> MKQECNVCYFNLPDPE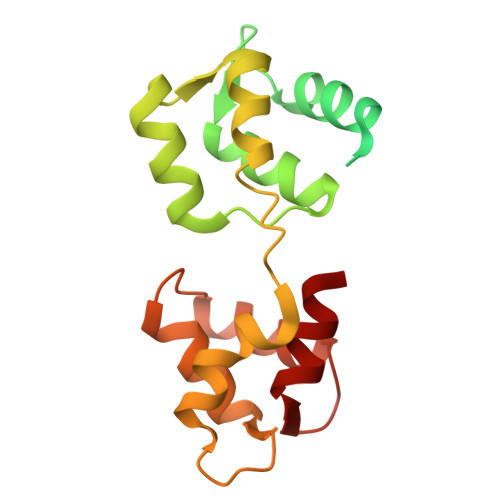STLGPYDNELNYFTWGPGFEYEPEPQRKPLSIEESFENSEESEESVADIQQLEEKVDESDVRIYFNEKSSGGKISIDNASYNARKLGLAPSSIDEKKIKELYGDNLTYEQYLEYLSICVHDKDNVEELIKMFAHFDNNCTGYLTKSQMKNILTTWGDALTDQEAIDALNAFSSEDNIDYKLFCEDILQ> MGW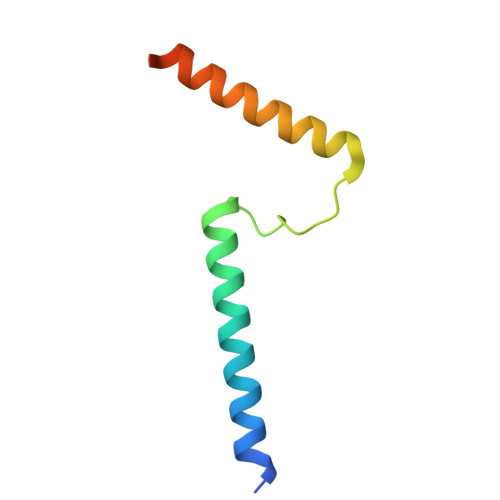YALPSYVIVSAAWAAGFWAIDTYQIYKEGKPSWNQNKDQFQRALYRRDWYLRREQETIGMFLGFDYGA> EFMVSLPRMVYPQPKVLTPCRKDVLVVTPWLAPIVWEGTFNIDILNEQFRLQNTTIGLTVFAIKKYVAFLKLFLETAEKHFMVGHRVHYYVFTDQPAAVPRVTLGTGRQLSVLEVRAYKRWQDVSMRRMEMISDFCERRFLSEVDYLVCVDVDMEFRDHVGVEILTPLFGTLHPGFYGSSREAFTYERRPQSQAYIPKDEGDFYYLGGFFGGSVQEVQRLTRACHQAMMVDQANGIEAVWHDESHLNKYLLR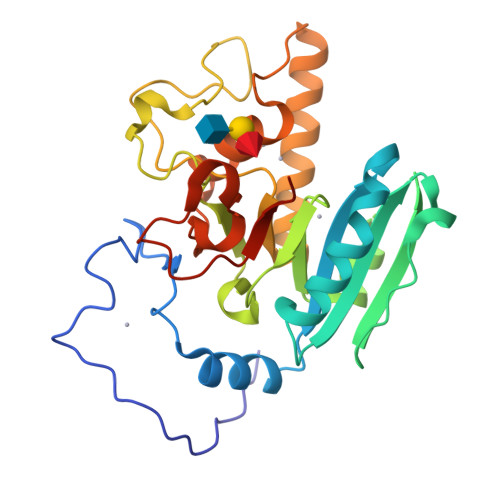HKPTKVLSPEYLWDQQLLGWPAVLRKLRFTAVPKNHQAVRNP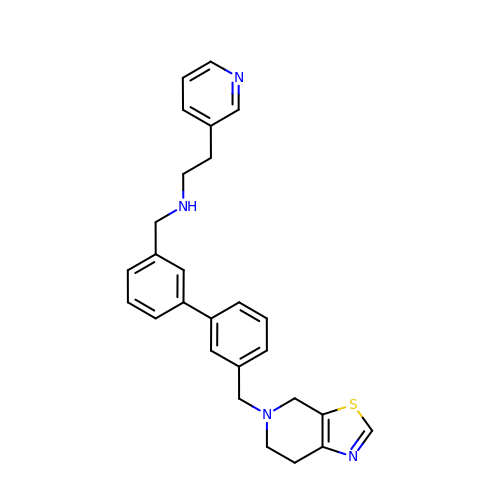N-[[3-[3-(6,7-dihydro-4H-[1,3]thiazolo[5,4-c]pyridin-5-ylmethyl)phenyl]phenyl]methyl]-2-pyridin-3-yl-ethanamine | C27 H28 N4 S | WPEZKMWVHQXQCY-UHFFFAOYSA-N> MGSSHHHHHHSAKETFYITTPIYYPSGNLHIGHAYSTVAGDVIARYKRMQGYDVRYLTGTDEHGQKIQEKAQKAGKTEIEYLDEMIAGIKQLWAKLEISNDDFIRTTEERHKHVVEQVFERLLKQGDIYLGEYEGWYSVPDETYYTESQLVDPQYENGKIIGGKSPDSGHEVELVKEESYFFNISKYTDRLLEFYDQNPDFIQPPSRKNEMINNFIKPGLADLAVSRTSFNWGVHVPSNPKHVVYVWIDALVNYISALGYLSDDESLFNKYWPADIHLMAKEIVRFHSIIWPILLMALDLPLPKKVFAHGWILMKDGKMSKSKGNVVDPNILIDRYGLDATRYYLMRELPFGSDGVFTPEAFVERTNFDLANDLGNLVNRTISMVNKYFDGELPAYQGPLHELDEEMEAMALETVKSYTESMESLQFSVALSTVWKFISRTNKYIDETTPWVLAKDDSQKDMLGNVMAHLVENIRYAAVLLRPFLTHAPKEIFEQLNINNPQFMEFSSLEQYGVLNESIMVTGQPKPIFP

Methionyl-tRNA synthetase (MetRS) charges tRNAMet with l-methionine (L-Met) to decode the ATG codon for protein translation, making it indispensable for all cellular lives. Many gram-positive bacteria use a type 1 MetRS (MetRS1), which is considered a promising antimicrobial drug target due to its low sequence identity with human cytosolic MetRS (HcMetRS, which belongs to MetRS2). The overall structure of SaMetRS resembles that of MetRS from other organisms, and it consists of a Rossmann fold aminoacylation domain (AD, residues 1–116 and 235–299), a connecting peptide (CP) domain (residues 117–234) inserted into the Rossmann fold, a stem contact fold (SCF) (residues 300–363), and a helical anticodon-binding domain (ABD) (residues 364–486). The CP domain of SaMetRS contains one single knuckle that lies on the top of the catalytic core, characterizing SaMetRS as MetRS1.

Recently, a series of phenylbenzimidazole inhibitors against SaMetRS were identified through DNA encoded library technology (DELT), and these inhibitors exhibited potent enzyme inhibition and moderate antibacterial activities. A representative compound (named P80 in our study) was synthesized, and its inhibitory activity against SaMetRS was measured. P80 inhibited the pretransfer editing activity of SaMetRS with IC50 = 94.6 ± 6.7 nM. We determined the crystal structure of SaMetRS with P80 at 1.92 Å resolution. As shown in its cocrystal structure with SaMetRS, the four branches of P80 stretched in different directions to interact with SaMetRS. As the first branch, the tert-butylbenzene segment lies on the L-Met binding site and forms extensive hydrophobic interactions with residues Pro11, Trp237, Ala240, Leu241, Tyr244, Ile273 and Phe276. Binding of this moiety to the L-Met site did not induce the Trp237 flip like what L-Met did, and maintained an open L-Met site, as observed in F- and A-state SaMetRS. As a result, the CP domain did not bend, keeping the auxiliary pocket in the open conformation. As the third branch, the bromobenzene moiety of P80 stretched deeply into the auxiliary pocket formed by residues Asp51, His54, Gly55, Glu55, Lys56, Ile57, Thr96 and Asp239 from AD and residues Val224 and Val234 from the CP domain. The benzimidazole group formed the fourth branch, and it extended toward the ATP phosphate group binding site.(2R)-2,3-bis(hexyloxy)propyl hydrogen (S)-pentylphosphonate | C20 H43 O5 P | 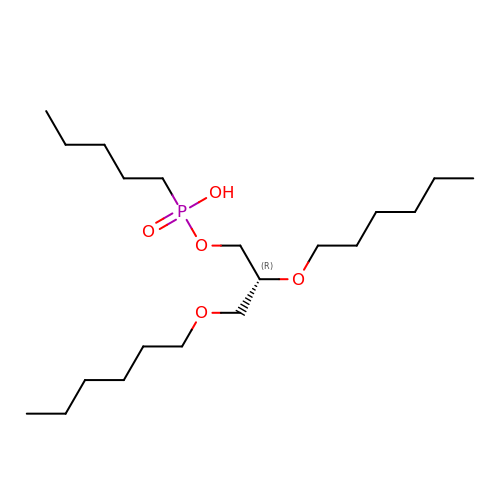PSVODCVMDBUUJZ-HXUWFJFHSA-N> MVNPFIKEAKEKMKRTLEKIEDELRKMRTGKPSPAILEEIKVDYYGVPTPVNQLATISISEERTLVIKPWDKSVLSLIEKAINASDLGLNPINDGNVIRLVFPSPTTEQREKWVKKAKEIVEEGKIAIRNIRREILKKIKEDQKEGLIPEDDAKRLENEIQKL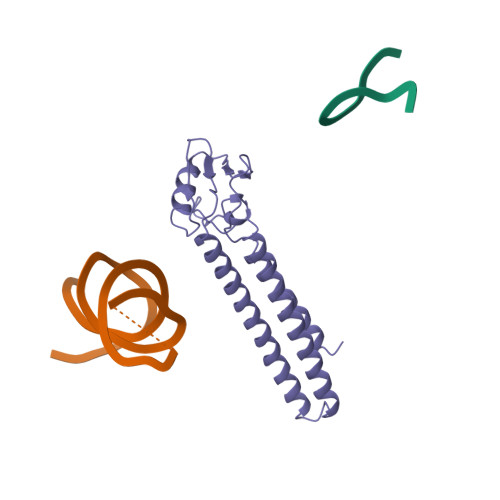TDEFIEKLDEVFEIKKEEIMEF> SNMLLNYVPVYVMLPLGV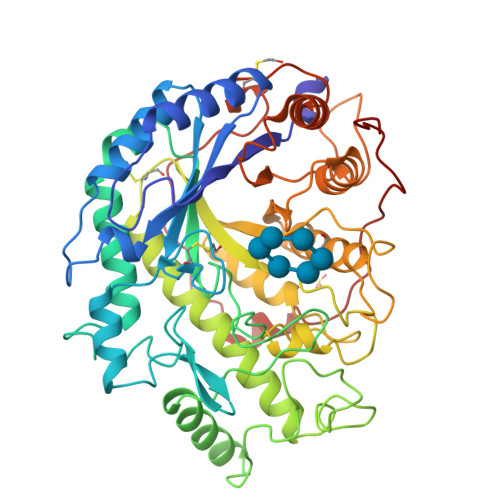VNVDNVFEDPDGLKEQLLQLRAAGVDGVMVDVWWGIIELKGPKQYDWRAYRSLFQLVQECGLTLQAIMSFHQCGGNVGDIVNIPIPQWVLDIGESNHDIFYTNRSGTRNKEYLTVGVDNEPIFHGRTAIEIYSDYMKSFRENMSDFLESGLIIDIEVGLGPAGELRYPSYPQSQGWEFPRIGEFQCYDKYLKADFKAAVARAGHPEWELPDDAGKYNDVPESTGFFKSNGTYVTEKGKFFLTWYSNKLLNHGDQILDEANKAFLGCKVKLAIKVSGIHWWYKVENHAAELTAGYYNLNDRDGYRPIARMLSRHHAILNFTCLEMRDSEQPSDAKSGPQELVQQVLSGGWREDIRVAGENALPRYDATAYNQIILNAKPQGVNNNGPPKLSMFGVTYLRLSDDLLQKSNFNIFKKFVLKMHADQDYCANPQKYNHAITPLKPSAPKIPIEVLLEATKPTLPFPWLPETDMKVDG>MSVVGTPKSAEQIQQEWDTNPRWKDVTRTYSAEDVVALQGSVVEEHTLARRGAEVLWEQLHDLEWVNALGALTGNMAVQQVRAGLKAIYLSGWQVAGDANLSGHTYPDQSLYPANSVPQVVRRINNALQRADQIAKIEGDTSVENWLAPIVADGEAGFGGALNVYELQKALIAAGVAGSHWEDQLASEKKCGHLGGKVLIPTQQHIRTLTSARLAADVADVPTVVIARTDAEAATLITSDVDERDQPFITGERTREGFYRTKNGIEPCIARAKAYAPFADLIWMETGTPDLEAARQFSEAVKAEYPDQMLAYNCSPSFNWKKHLDDATIAKFQKELAAMGFKFQFITLAGFHALNYSMFDLAYGYAQNQMSAYVELQEREFAAEERGYTATKHQREVGAGYFDRIATTVDPNSSTTALTGSTEEGQFHLEHHHHHH[2x]

Isocitrate lyases (ICLs; isoforms 1 and 2) catalyze the reversible conversion of isocitrate to glyoxylate and succinate in the glyoxylate cycle, which is used to bypass the two decarboxylation steps of the tricarboxylic acid (TCA) cycle. The ICL-initiated glyoxylate cycle is essential for various organisms, including bacteria, fungi, and plants, to reactivate the TCA cycle in circumstances that limit carbon supply as an energy source by offering alternative energy sources such as fatty acids. Owing to the crucial function of ICLs for the survival of M. tuberculosis in the host, they have been considered major therapeutic targets for the treatment of tuberculosis. Although it has been shown that itaconate produced by a host directly inhibits an ICL from M. tuberculosis (tbICL) to protect against the infection, the molecular mechanism of ICL inhibition by itaconate remains elusive.

Among the crystals prepared using various combinations of substrates and itaconate, the structure of tbICL in complex with succinate and itaconate was determined at 2.58 Å resolution. The crystal belongs to space group P6522, with two molecules (subunits A and B) present in the asymmetric unit. In our structure, succinate (a substrate/product of tbICL) and itaconate (an inhibitor of tbICL) were bound to the active sites of chains A and B, respectively. Thus, although each subunit contains a different molecule in the active site, this distribution of heterogeneous molecules in the two subunits did not cause significant structural differences. In the active site of subunit A, two carboxylic acid groups of succinate are coordinated to adjacent water molecules, by which interactions with residues such as Ser91, Trp93, Asp108, Asp153, Glu182, Arg228, Glu285, Asn313, and Thr347 are mediated. However, itaconate directly interacts electrostatically with proximal residues, such as Arg228 and Asn313, whereas succinate does so only with Arg228. In addition, while succinate directly binds to five water molecules, itaconate directly interacts with only three water molecules. These differences suggest that itaconate is relatively less dependent on water molecules for binding to the active site than succinate is. However, we found that the positions of the L5 loop (residues 189–197) and the C-terminal tail are different, depending on the conformer. Moreover, our structure corresponds to the same open form as that observed in the native form, although subunit B has the inhibitor itaconate in the active site. Based on these results, we assume that the incorporation of heterogeneous compounds into their respective active sites induces subtle movements of nearby residues, thereby generating abnormal electric fields and finally obstructing active site closure.> GNPFEGVQLWANNYYRSEVHTLAIPQITDPALRAAASAAAEVPSFLWLDTLDKTPLMEQTLADIRTANKNGGNYAGQFVVYD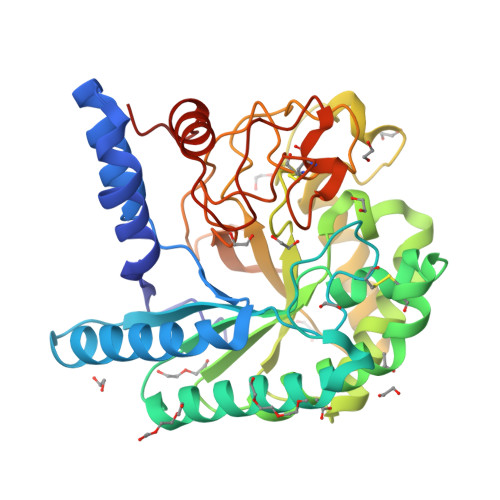LPDRDCAALASNGEYSIADGGVAKYKNYIDTIRQIVVEYSDIRTLLVIEPDSLANLVTNLGTPKCANAQSAYLECINYAVTQLNLPNVAMYLDAGHAGWLGWPANLDPAAQLFANVYKNASSPRALRGLATNVANYNAWSIASPPPYTSPNPNYDEKHYIEAFAPLLRNQGFDAKFIVDTGRNGKQPTGQLEWGHWCNVKGTGFGVRPTANTGHELVDAFVWVKPGGESDGTSDPSAPRFDPHCALPDALQPAPQAGAWFQAYFVQLLTNANPSFLHHHHHH>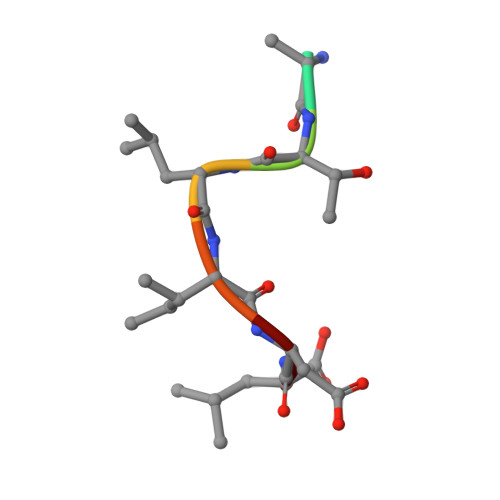 GYTLIDL>GSPKDPKRIAVVAPTYAGGLKKLGANIVAVNQQVDQSKVLKDKFKGVTKIGDGDVEKVAKEKPDLIIVYSTDKDIKKYQKVAPTVVVDYNKHKYLEQQEMLGKIVGKEDKVKAWKKDWEETTAKDGKEIKKAIGQDATVSLFD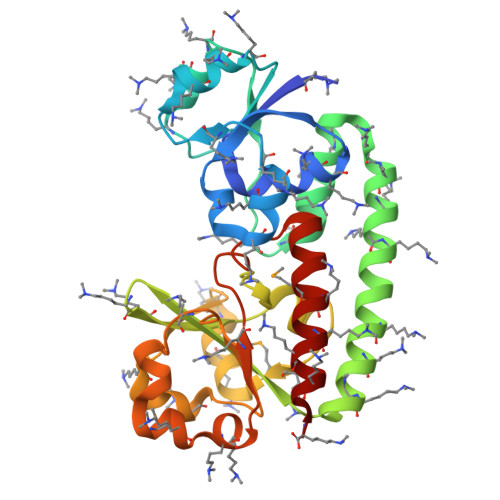EFDKKLYTYGDNWGRGGEVLYQAFGLKMQPEQQKLTAKAGWAEVKQEEIEKYAGDYIVSTSEGKPTPGYESTNMWKNLKATKEGHIVKVDAGTYWYNDPYTLDFMRKDLKEKLIKAAK[2x]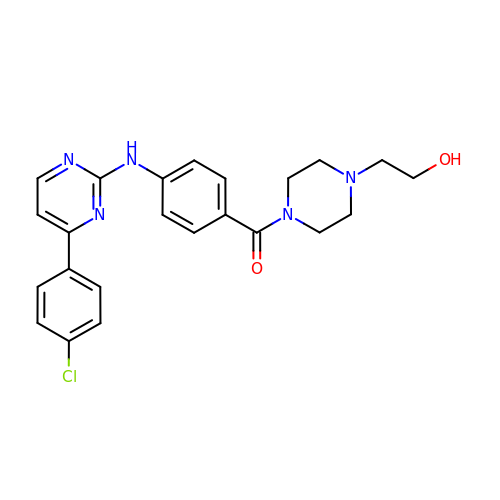(4-{[4-(4-chlorophenyl)pyrimidin-2-yl]amino}phenyl)[4-(2-hydroxyethyl)piperazin-1-yl]methanone | C23 H24 Cl N5 O2 | HMSMXFYWPQNMCE-UHFFFAOYSA-N> MSFTNATFSQVLDDLSARFILNLPAEEQSSVERLCFQIEQAHWFYEDFIRAQNDQLPSLGLRVFSAKLFAHCPLLWKWSKVHEEAFDDFLRYKTRIPVRGAIMLDMSMQQCVLVKGWKASSGWGFPKGKIDKDE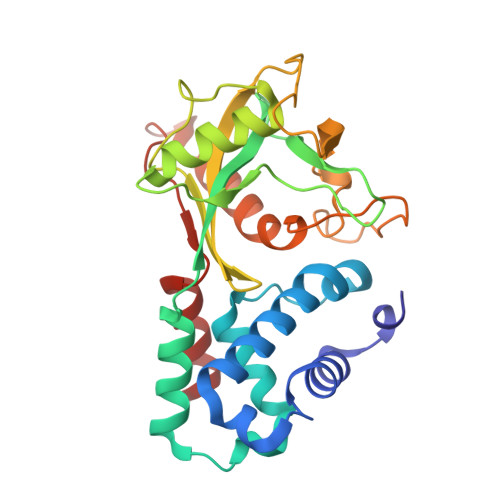SDVDCAIREVYEETGFDCSSRINPNEFIDMTIRGQNVRLYIIPGISLDTRFESRTRKEISKIEWHNLMDLPTFKKNKPQTMKNKFYMVIPFLAPLKKWIKKRNIANNTTKEKNISVDVDADASSQLLSLLKS Pur-alpha is an ubiquitously expressed, multifunctional protein that binds to both DNA and RNA and is known to regulate replication, transcription, and translation. It has been shown that Pur-alpha binds to single- and double-stranded nucleic acids that contain GGN motifs. Nucleic acid-binding of Pur-alpha is mediated by three central PUR repeats, which are N-terminally flanked by unstructured, glycine-rich sequences and C-terminally by glutamine- and glutamate-rich regions (Johnson et al., 2013). Besides its ability to bind RNA and DNA, Pur-alpha possesses dsDNA-destabilizing activity in an ATP-independent fashion.

To understand the role of the third repeat of Pur-alpha for DNA/RNA binding, we determined its crystal structure. The final structure model was obtained in the same way from selenomethionine-derivatized crystals at 2.6 Å resolution. Two molecules (one depicted in brown, the other in yellow) of repeat III form a dimer with intertwined α-helices, very similar to Pur-alpha repeat I-II. PUR repeat III was previously suggested to mainly mediate dimerization of Pur-alpha. We therefore performed EMSA and observed that Pur-alpha repeat III bound with weaker affinities to CGG repeats and to MF0677 than Pur-alpha repeat I-II. Also in fluorescence-polarization experiments, PUR repeat III bound MF0677 ssDNA over 30-times weaker than PUR repeat I-II. Although Pur-alpha repeat III does not have a phenylalanine in the corresponding position of F145 of PUR repeat II, it also contains a conserved aromatic residue (Y219), which could potentially undergo stacking with DNA bases and support dsDNA unwinding. However, in unwinding assays almost no activity was observed for PUR repeat III. These observations confirm that PUR repeats I-II mediate the main nucleic-acid-binding and unwinding activities and suggest that repeat III might predominantly mediate dimerization. Since in the crystal structure the C-terminal end of PUR repeat I-II is located on the opposite side of its nucleic-acid-binding surface (bottom), it is unlikely that PUR repeat III causes steric clashes interfering with the nucleic-acid binding by PUR repeat I-II.

>GPLGSDGGRFKGDLPEERHMKVDNKNFYFDIGQNNRGVYMRISEVKNNFRTSITIPEKCWIRFRDIFNDYCEKMKKSSDSI[6x]>MLYYVSILLMAVYAVAVADEDPMTCDKLPKVPVPPLEEFIKSNPLQFAYVLTDT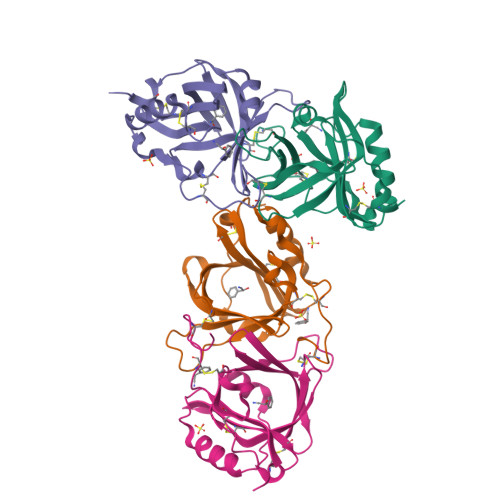FDCTTRVYVQPARLSPNQAATALDIRGSRIITNDFVGGPNNSAILNNCTTGEKATWYFQYTNLNTPNGSSYCAYTCNGEEIAEYKCANNNNGTDPLQKQAVEVAKKVPNGDKIHYALDNCPEHHGCFAFY[4x]>VVCSLCKREGHLKKDCPEDFKRIQLEPLPPLTPKFLNILDQVCIQCYKDFSPTIIEDQAREHIRQNLESFIRQDFPGTKLSLFGSSKNGFGFKQSDLDVCMTINGLETAEGLDCVRTIEELARVLRKHSGLRNILPITTAKVPIVKFFHLRSGLEVDISLYNTLALHNTRLLSAYSAIDPRVKYLCYTMKVFTKMCDIGDASRGSLSSYAYTLMVLYFLQQRNPPVIPVLQEIYKGEKKPEIFVDGWNIYFFDQIDELPTYWSECGKNTESVGQLWLGLLRFYTEEFDFKEHVISIRRKSLLTTFKKQWTSKYIVIEDPFDL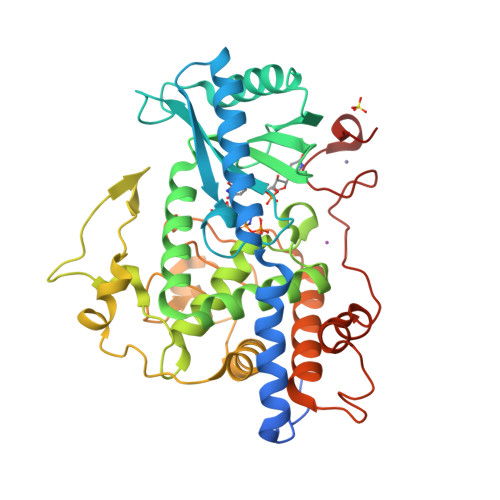NHNLGAGLSRKMTNFIMKAFINGRRVFGIPVKGFPKDYPSKMEYFFDPDVLTEGELAPNDRCCRICGKIGHFMKDCPMRRK[3x]>MGQVGRQLAIIGDDINRRYDSEFQTMLQHLQPTAENAYEYFTKIATSLFESGINW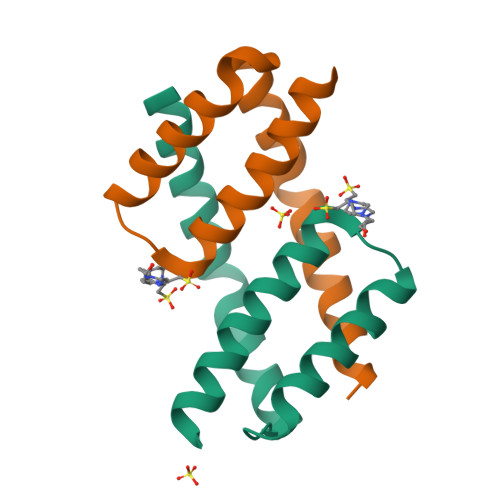GRVVALLGFGYRLALHVYQHGLEENLYFQ[6x]Clostridium thermocellum has extensive potential in lignocellulose biorefineries as an environmentally prominent, thermophilic, cellulolytic bacterium. Previously, five putative sugar transporters, denoted A to D and L and belonging to the ABC transport systems group, were identified in the genome of C. thermocellum, and the solute-binding lipoproteins (SBP) of these ABC transporters were shown to bind different dextrins by isothermal titration calorimetry (ITC) assays. To gain insight into the structural mechanism of the transporter specificities, 11 crystal structures, both alone and in complex with appropriate saccharides, were solved for all 5 putative sugar-binding proteins, thus providing detailed specific interactions between the proteins and the corresponding saccharides. Combined genetic, biophysical, and structural studies have provided solid evidence that transporter A and transporter B are the major glucose and cellodextrin transporters, respectively, among the five potential sugar transporters in C. thermocellum.

The unliganded CbpC and CbpD structures were determined to 2.00 and 1.50 Å resolution, respectively. A Dali search using the CbpC structure revealed similarities with several sugar- and other solute-binding proteins of ABC transporters. However, the expected substrate-binding pocket between domain I and domain II in CbpC was blocked by an additional loop that was absent in the other proteins, suggesting that CbpC might not be a functional sugar-binding protein. For CbpC and CbpD, no interaction was detected for all of the tested carbohydrate substrates in both ITC and NMR experiments, suggesting that transporters C and D are not responsible for glucose or cellodextrin transport. However, regardless of the exact specificity of CbpC and CbpD, the knockout mutants of these associated transporters clearly indicate that they do not play a significant role in the utilization of cellulose by C. thermocellum.

>[2x]SSGSRDDTQDVIGGKIVMYAAPGDNVQSEIRNIVRSKYPNVEFQVVSFNNADEFKSRLLTELMAGEGPDVIVLSPSTKKGSITIETMRKLVESGVFCDLEPYISKDESINLSEYNETVLNSGVINGKRYFIPIAYDVPIFWTANSILEENNIKDEIANWTLKDMADFAVQFKEKNSDNYLFGYGDGFIRNIMYANWREFVDYENKQASFDSQEFVEFLEAIGAIEKAGICDEKLIKEYTGMEFEALKHGKITLISSTEYPINPWELWYRNSHINYYFNPDSIRLSKFPTFGDLGRIVAHPTDIVAINKNSKNKATAYEVLKVFLSKEIQSSQQFRDRMGIPVNDEAIRELIEKYSGEEGKTTLPVGMTINETMDTVPLPESVVAEYNSIINGVTECVLVDEQIIDFMIEGFNEYKNGKMSAKDAARMVQQKVNLFLNE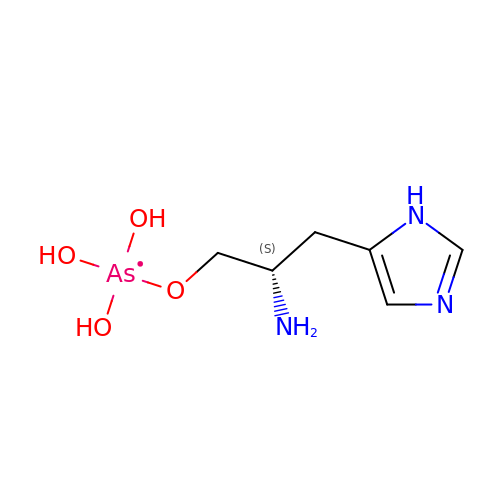{[(2S)-2-amino-3-(1H-imidazol-5-yl)propyl]oxy}(trihydroxy)-lambda~5~-arsanyl | C6 H13 As N3 O4 | ULOXOLOOGPGSSX-YFKPBYRVSA-N> QYPIINFTTAGATVQSYTNFIRAVRG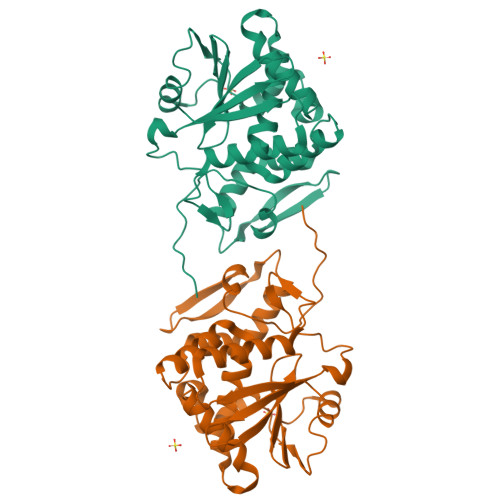RLTTGADVRHEIPVLPNRVGLPINQRFILVELSNHAELSVTLALDVTNAYVVGYRAGNSAYFFHPDNQEDAEAITHLFTDVQNRYTFAFGGNYDRLEQLAGNLRENIELGNGPLEEAISALYYYSTGGTQLPTLARSFIICIQMISEAARFQYIEGEMRTRIRYNRRSAPDPSVITLENSWGDLSTAIQESNQGAFASPIQLQRRNGSKFSVYDVSILIPIIALMVYRCAPPPSSQF> QPSFRPSALVVPVKKDASTLQYVTTINQRTPLVSENLVVDLGGRFLWVDCDQNYVSSTYRPVRCRTSQCSLSGSIACGDCFNGPRPGCNNNTCGVFPENPVINTATGGEVAEDVVSVESTDGSSSGRVVTVPRFIFSCAPTSLLQNLASGVVGMAGLGRTRIALPSQFASAFSFKRKFAMC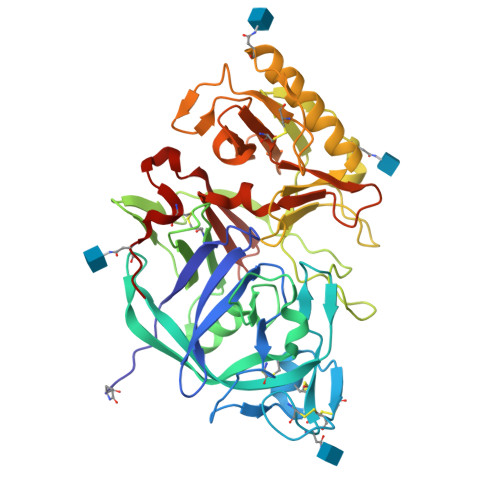LSGSTSSNSVIIFGNDPYTFLPNIIVSDKTLTYTPLLTNPVSTSATSTQGEPSVEYFIGVKSIKINSKIVALNTSLLSISSAGLGGTKISTINPYTVLETSIYKAVTEAFIKESAARNITRVASVAPFGACFSTDNILSTRLGPSVPSIDLVLQSESVVWTITGSNSMVYINDNVVCLGVVDGGSNLRTSIVIGGHQLEDNLVQFDLATSRVGFSGTLLGSRTTCANFNFTS> STQAATASSRNSCAADDKATEPLPKDCPVSSYNEWDPLEEVIVGRAENACVPPFTIEVKANTYEKYWPFYQKQGGHYFPKDHLKKAVAEIEEMCNILKTEGVTVRRPDPIDWSLKYKTPDFESTGLYSAMPRDILIVVGNEIIEAPMAWRSRFFEYRAYRSIIKDYFHRGAKWTTAPKPTMADELYNQDYPIHSVEDRHKLAAQGKFVTTEFEPCFDAADFIRAGRDIFAQRSQVTNYLGIEWMRRHLAPDYRVHIISFKDPNPHIDATFNIIGPGIVLSNPDRPCHQIDLFKKAGWTIITPPTPIIPDDHPLWMSSKWLSMNVLMLDEKRVMVDANEVPIQKMFEKLGITTIKVNIRNANSLGGGFHCWTCD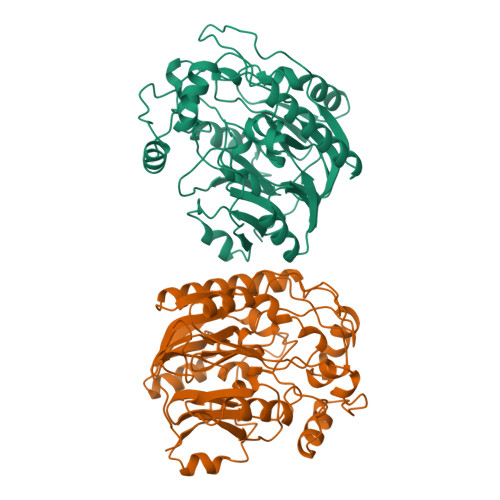VRRRGTLQSYLD~{N}-[(2-azanyl-3~{H}-1,3-benzothiazol-6-yl)methyl]-1~{H}-indole-2-carboxamide 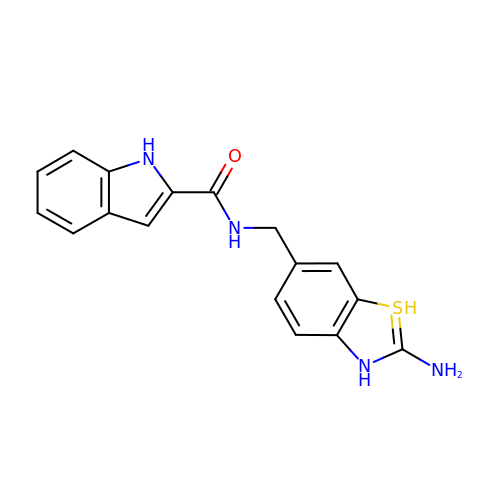| C17 H16 N4 O S | GAUGHKFDIIXTPX-UHFFFAOYSA-N>YLEAFPKELREYYKNLFGKEEANKIMKKLREPVEHYYIRVNTLKISREKLIGELKKEGLKPLRSPYLPEGLYFVREGPNFSDDFEPKLPVVVANKYAAESVYQGAMLYAPGVLKADKNIKEGDEVQIRDPKGLLVGIGIARMDYKEMTEATRGLAVEVTLPKFKLPSLSELKAFEKGYFYPQGLPSMVTARVLEPKEDDVIIDMAAAPGGKTTHIAQLLENKGEIIAIDKSKNRLRKMEENIKRLGVKNVKLVQMDARKLPDLGIKADKILLDAPCTALGVRPKLWEERTLKHIEATARYQRAFIWAAIKSLRRGGVLVYSTCTLSYEENEGNVKFMIRKGMKLEEQSIFIGSPGIGMNKVQRFYPHKHLTQGFFIAKLRKVKD[2x]

In this study, we identified that PH1991 is a tRNA:m5C72 MTase NSun6 (PhNSun6). In contrast to hNSun6, which could only methylate four tRNAs with U73, PhNSun6 could catalyze m5C72 formation on eleven PhtRNAs harboring either U73 or G73. PhNSun6, with 12 α-helices and 19 β-strands, is divided into two distinct domains with different sizes: the MTase domain, including an RRM motif (residues 34–79 and residues 173–185) and a Rossmann-fold catalytic core (residues 185–389), and the PUA domain (residues 86–164). The tRNA substrates recognized by PhNSun6 were based on (i) the 3′ CCA terminus, (ii) the target site C72, (iii) U73 or G73, and (iv) the discriminatory base pair C2:G71 at the acceptor stem.

To fully decipher the RNA recognition mechanism of PhNSun6, we obtained the crystal structures of PhNSun6 with and without its cofactors, including apo-PhNSun6, and PhNSun6 complexed with SAM, SFG and SAH, which diffracted to 2.6, 2.5, 2.5 and 2.2 Å, respectively. The PUA domain is inserted into the MTase domain via two linkers: Residues 79–86 and residues 164–173. A non-conserved extension motif (residues 1–34) was observed at the N-terminus. When comparing the structures of PhNSun6 in the apo form and in the form bound with cofactors, the overall structures do not show distinct changes, except that helix α9 moves a slightly toward the cofactors. Although PhNSun6 contains a different RNA recognition motif compared with that in hNSun6, the main structure of PhNSun6 adopts a similar topology to hNSun6 and the two active Cys residues of PhNSun6 are conserved. Some structural differences were observed between PhNSun6 and hNSun6. Second, for the PUA domain, most important difference concerns the change in the orientations of PhNSun6 helix α4 and hNSun6 α5. Third, PhNSun6 lacks the eukaryotic specific Lys-rich loop. Taken together, the structural differences between PhNSun6 and hNSun6 might contribute to the distinct tRNA substrate recognition mechanisms.> GRPLLQA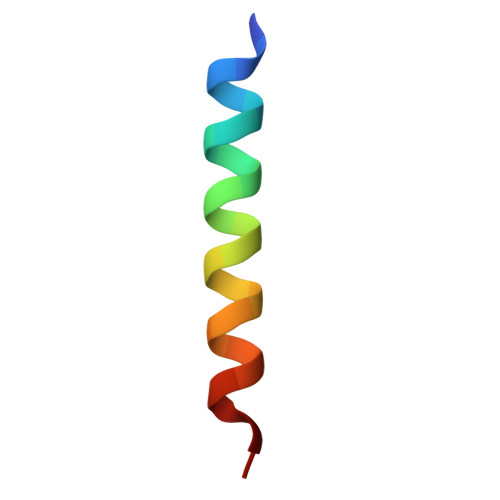AKGLAGAVSELLRSAQP>[4x]TPKPKIVLVGS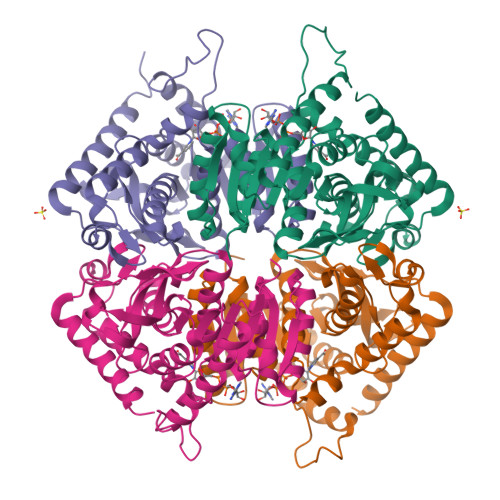GMIGGVMATLIVQKNLGDVVMFDVVKNMPQGKALDTSHSNVMAYSNCKVTGSNSYDDLKGADVVIVTAGFTKAPGKSDKEWNRDDLLPLNNKIMIEIGGHIKNLCPNAFIIVVTNPVDVMVQLLFEHSGVPKNKIIGLGGVLDTSRLKYYISQKLNVCPRDVNALIVGAHGNKMVLLKRYITVGGIPLQEFINNKKITDEEVEGIFDRTVNTALEIVNLLASPYVAPAAAIIEMAESYLKDIKKVLVCSTLLEGQYGHSNIFGGTPLVIGGTGVEQVIELQLNAEEKTKFDEAVAETKRMKALIHHHHHH> NATEIRASVGKMIDGIGRFYIQMCTELKLSDYEGRLIQNSLTIERMVLSAFDERRNKYLEEHPSAGKDPKKTGGPIYRRVDGKWRRELILYDKEEIRRIWRQANNGDDATAGLTHMMIWHSNLNDATYQRTRALVRTGMDPRMCSLMQGSTLPRRSGAAGAAVKGVGTMVMELIRMIKRGINDRNFWRGENGRRTRIAYERMCNILKGKFQTAAQRTMVDQVRESRNPGNAEFEDLIFLARSALILRGSVAHKSCLPACVYGSAVASGYDFEREGYSLVGIDPFR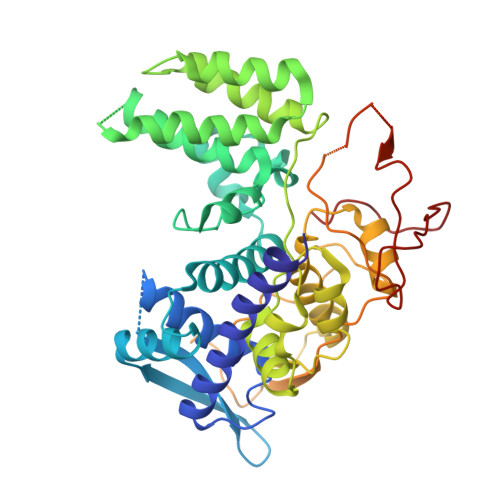LLQNSQVYSLIRPNENPAHKSQLVWMACHSAAFEDLRVSSFIRGTKVVPRGKLSTRGVQIASNENMETMESSTLELRSRYWAIRTRSGGNTNQQRASSGQISIQPTFSVQRNLPFDRPTIMAAFTGNTEGRTSDMRTEIIRLMESARPEDVSFQGRGVFELSDEKATSPIVPSFDMSNEGSYFF>[2x]GTSMETFDPTELPELLKLYYRRLFPYSQYYRWLNYGGVIKNYFQHREFSFTLKDDIYIRYQSFNNQSDLEKEMQKMNPYKIDIGAVYSHRPNQHNTVKLGAFQAQEKELVFDIDMTDYD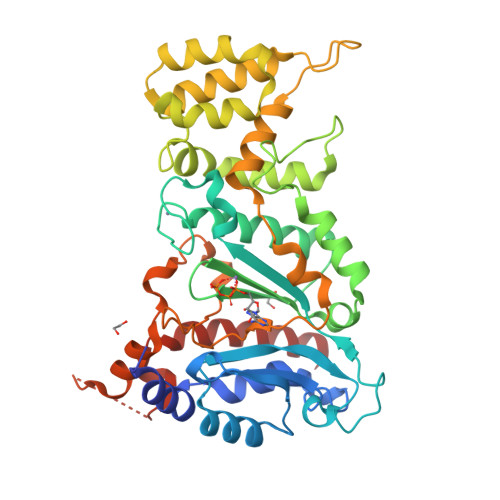DVRRCCSSADICPKCWTLMTMAIRIIDRALKEDFGFKHRLWVYSGRRGVHCWVCDESVRKLSSAVRSGIVEYLSLVKGGQDVKKKVHLSEKIHPFIRKSINIIKKYFEEYALVNQDILENKESWDKILALVPETIHDELQQSFQKSHNSLQRWEHLKKVASRYQNNIKNDKYGPWLEWEIMLQYCFPRLDINVSKGINHLLKSPFSVHPKTGRISVPIDLQKVDQFDPFTVPTISFICRELDAISTNEEEKEENEAESDVKHRTRDYKKTSLAPYVKVFEHFLENLDKSRK> ATLDSWLSNEATVARTAILNNIGADGAWVSGADSGIVVASPSTDNPDYFYTWTRDSGLVIKTLVDLFRNGDTDLLSTIEHYISSQAIIQGVSNPSGDLSSGGLGEPKFNVDETAYTGSWGRPQRDGPALRATAMIGFGQWLLDNGYTSAATEIVWPLVRNDLSYVAQYWNQTGYDLWEEVNGSSFFTIAVQHRALVEGSAFATAVGSSCSWCDSQAPQILCYLQSFWTGSYILANFDSSRSGKDTNTLLGSIHTFDPEAGCDDSTFQPCSPRALANHKEVVDSFRSIYTLNDGLSDSEAVAVGRYPEDSYYNGNPWFLCTLAAAE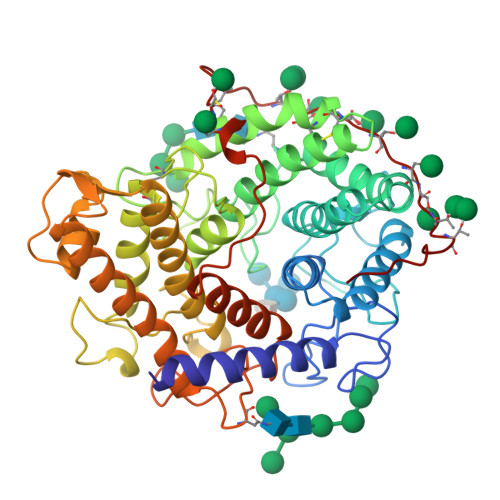QLYDALYQWDKQGSLEITDVSLDFFKALYSGAATGTYSSSSSTYSSIVSAVKTFADGFVSIVETHAASNGSLSEQFDKSDGDELSARDLTWSYAALLTANNRRNSVVPPSWGETSASSVPGTCAATSASGTYSSVTVTSWPSIVAT>[6x]MHSGIDIRVARPEDAEEIQIIYAPIVLNTAISFEEAVPSVEQMRERISTTLQTYPYLVAVREGRVVGYAYASQHRARAAYRWAVDVTVYVAEGQRRSGIARQLYDVLL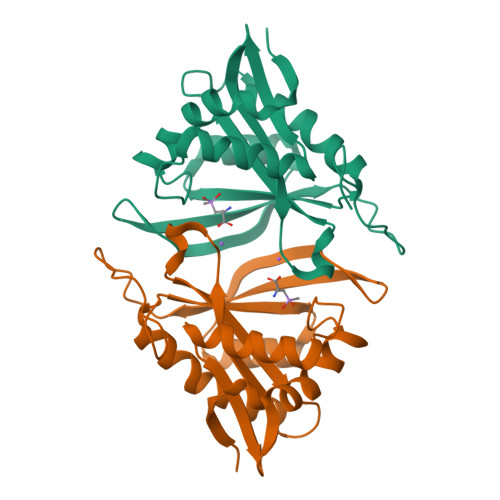PVLKRLGYRSAYAGIALPNEGSVGLHERLGFQHIGTFPQVGFKLDAWHDVGYWRFDFGDEGLHPEAPLGFLSQIPLGPEQKLISEEDLNSAVDHHHHHH2-chloro-4-{[(1R,2R)-2-hydroxy-2-methylcyclopentyl]amino}-3-methylbenzonitrile | C14 H17 Cl N2 O | 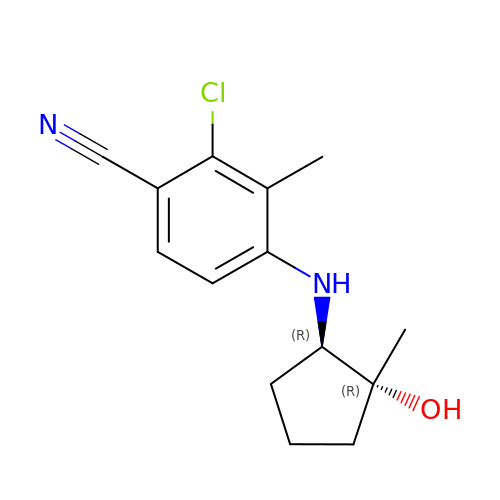CXFSVKGROITHRY-TZMCWYRMSA-N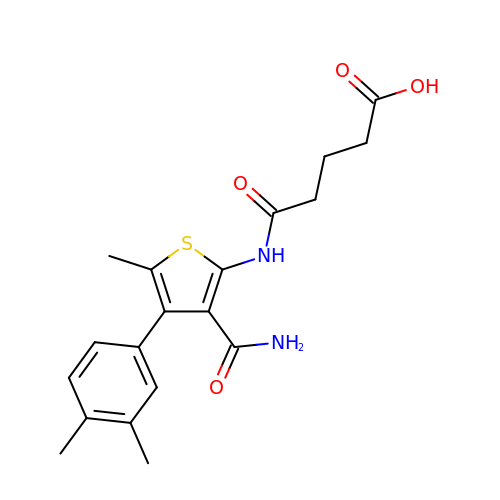5-{[3-carbamoyl-4-(3,4-dimethylphenyl)-5-methylthiophen-2-yl]amino}-5-oxopentanoic acid | C19 H22 N2 O4 S | ZOPDRGUNCASWKP-UHFFFAOYSA-N> GLTYCTHASGFSFNPQTADAGTSMNVVTEQIYNKLFDIKNHSATLTPMLAQSYSISADGKEILLNLRHGVKFHQTPWFTPTRDFNAEDVVFSINRVLGHNTYLPTLAEANVTYSNPQYKVFHEQARKVRFPYFDSIKLNEKIKSVTALSPYQVKIELFAPDSSILSHLASQYAIIFSQEYAYQLSADDNLAQLDTHPVGTGPYQVKDYVYNQYVRLVRNENYWKKEAKIEHIIVDLSTDRSGRLVKFFNNECQIASYPEVSQIGLLKNDDKHYYMQSTDGMNLAYLAFNFDKPLMRDHEIRAAISQSLNRARIIHSIYHNTATVANNIIPEVSWASTVNTPEFEFDYHPKIAKNKLADKNLLLNLWVINEEQVYNPAPFKMAEMIKWDLAQAGVKVKVRAVTRPFLTAQLRNQSENYDLILSGWLAGNLDPDGFMRPILSCGTKNELTNLSNWCNEEFDQFMDRAITTSHLSSRAKAYNEAQELVLRELPIIPIANVKRILVANSRVKGVKMTPFGSLDFS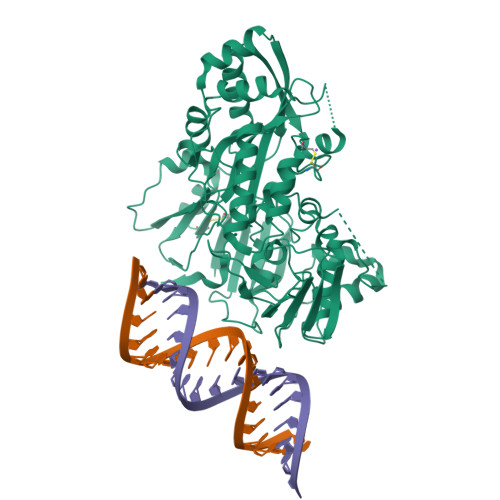TLYFI2-[(5-CHLORO-2-PYRIDYL)SULFANYL]ETHANOL | C7 H8 Cl N O S | 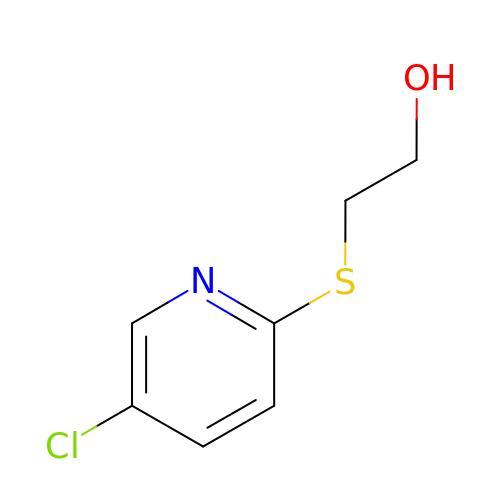KLOJLJIHCJJDCT-UHFFFAOYSA-N> VVVVVVVVVVVVVVVVVVV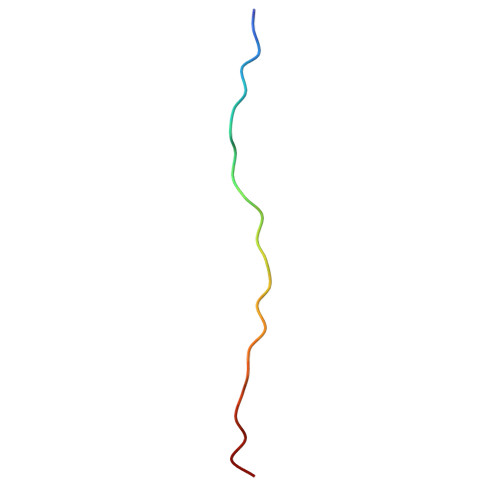VVVV> KGKSEVVEQNHTLILGWSDKLGSLLNQLAIANESLGGGTIAVMAERDKEDMELDIGKMEFDFKGTSVICRSGSPLILADLKKVSVSKARTIIVLAEDGNADQSDARALRTVLSLTGVKEGLRGHIVVEMSDLDNEVLVKLVGGDLVETVVAHDVIGRLMIQCARQPGLAQIWEDILGFENCEFYIKRWPQLDGMLFEDVLISFPAAIPCGIKVASYGGKIILNPDDSYVLQEGDEVLVIAEDDDTYAPAPLPMVRRGSLPKDFVYPKSPERILFCGWRRDMEDMITVLDASLAPDSELWMFNDVPEKEREKKLIDGGLDISRLENISLVNREGNAVIRRHLESLPLESFDSILILADESVEDSAIQADSRSLATLLLIRDIQARRLPYVAMASQTQGGNFSKGSWIGEMKQASDKTVIISEILDPRTKNLLSMSKISDYVLSNELVSMALAMVAEDRQINDVLEELFAEEGNEMHIRQADIYLREGEEMSFYEIMLRARQRREILIGYRLANAERAVINPPAKTGRRKWSLKDVFVVITEKE

Two DMI1 homologs, named POLLUX and CASTOR, were identified in L. japonicus and both of them are required to initiate symbiosis. To address these fundamental issues that define the primary function of these channels and their role in the symbiotic process, we performed functional characterization of the LjCASTOR channel and demonstrate that it functions as a Ca2+-regulated Ca2+ channel rather than as a K+ channel as previously proposed. We also determined the high-resolution crystal structure of the ligand-binding soluble domain of LjCASTOR and reveal that the entire soluble domain consists of two tandem RCK domains that assemble into a tetrameric gating ring where Ca2+ can bind and regulate the channel. Our high-resolution structure reveals multiple Ca2+-binding sites in the RCK gating ring and provides structural insights into Ca2+-regulated gating of CASTOR.

Other than one carboxylate oxygen atom from E493, which is also shared with the Ca(II) site, the rest of the Na+ ligands are all from backbone carbonyls of D485, G488, E490, and C492. The Na+ site is not Na+ specific as the structure determined by using crystals grown in the presence of KCl instead of NaCl demonstrated that K+ could also bind. Interestingly, K+ binding triggers some local structural changes, most notably the flip of the backbone carbonyl of L487, resulting in two additional oxygen ligands for K+ from the backbone carbonyls of I486 and L487. The K+ position is also slightly shifted from the Na+ site, resulting in longer ion–ligand distances in the range of 2.6–3.0 Å. It is intriguing to note that Na+ and K+ can modulate the open probability of the channel. With the same cytosolic [Ca2+], the channel has higher open probability in KCl than in NaCl. As this monovalent site is proximal to the Ca(II) site and also shares the same oxygen ligand from E493, we suspect that Na+ and K+ binding can exert a different competing effect on Ca2+ affinity and thereby have different modulation effect on Ca2+ activation.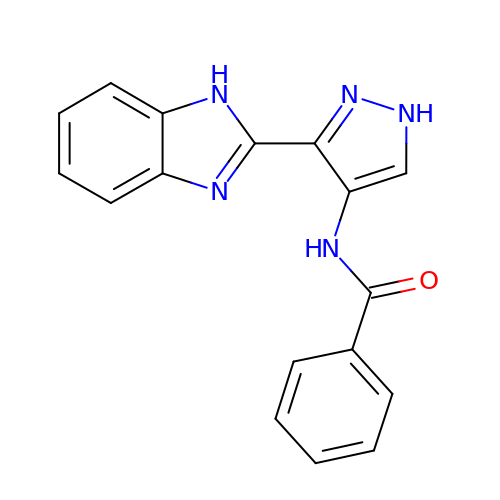N-[3-(1H-BENZIMIDAZOL-2-YL)-1H-PYRAZOL-4-YL]BENZAMIDE | C17 H13 N5 O | FPKSFXFWECAIBR-UHFFFAOYSA-N> SNAMAHSAEPTTEASRILIH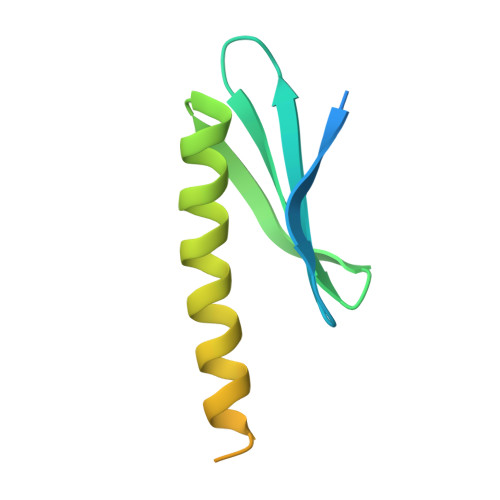SDARYEAFTVDLDYMWRWEILRDGEFVQEGCSLSFDSSRKAVAHVLSHFKRQDEAAQRPGDNSAEIKRLLQSLGTPIPVNEQNDSTKNELAQPE>MGSSHHHHHHSNDPMSRQANRGTESKKMSSELFTLTYGALVTQLCKDYENDEDVNKQLDKMGFNIGVRLIEDFLARSNVGRCHDFRETADVIAKVAFKMYLGITPSITNWSPAGDEFSLILENNPLVDFVELPDNHSSLIYSNLLCGVLRGALEMVQMAVEAKFVQDTLKGDGVTEIRMRFIRRIEDNLPAGEE[2x];>[2x]MADEALFLLLHNEMVSGVYKSAEQGEVENGRCITKLENMGFRVGQGLIERFTKDTARFKDELDIMKFICKDF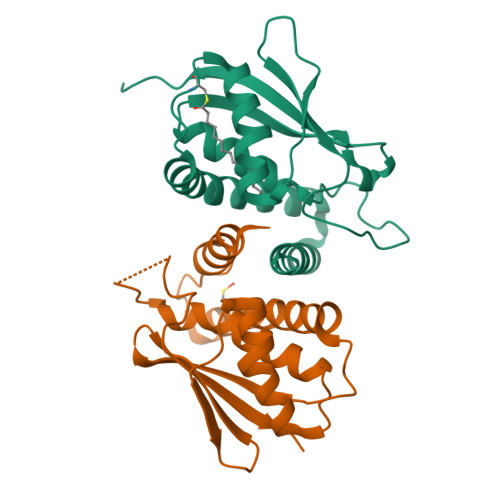WTTVFKKQIDNLRTNHQGIYVLQDNKFRLLTQMSAGKQYLEHASKYLAFTCGLIRGGLSNLGIKSIVTAEVSSMPACKFQVMIQKL(2R)-2-{4-[(3,5-dichloropyridin-2-yl)oxy]phenoxy}propanoic acid | C14 H11 Cl2 N O4 | 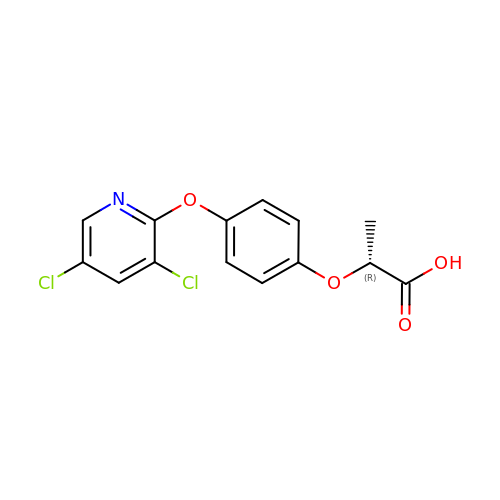SVGBNTOHFITEDI-MRVPVSSYSA-N>GGACTTCGCG[3x];>[3x]CGCG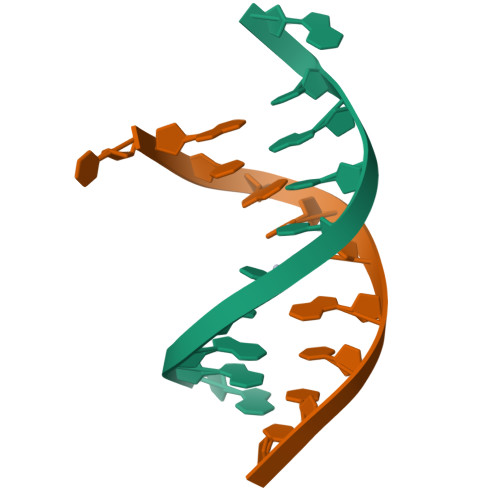TTGTCC7-[2-[3-(3-fluorophenyl)propylamino]ethyl]quinolin-2-amine | C20 H22 F N3 | 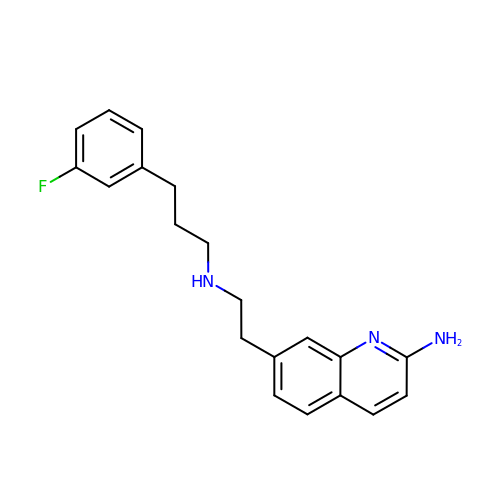ZCQVAHWJMSLTRU-UHFFFAOYSA-N> GNE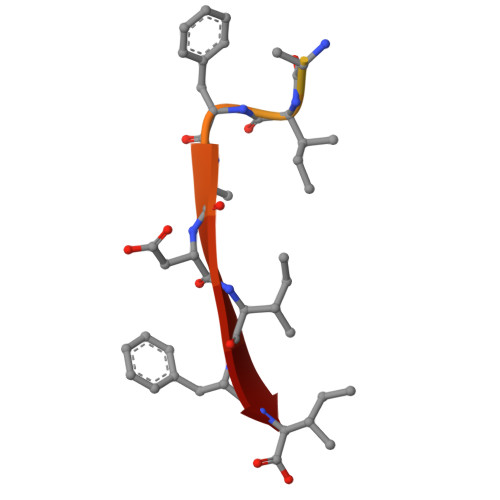EEEEDDGDIFADIFI>MRIPLVGKDSIESKDIGFTLIHEHLRVFSEAVRQQWPHLYNEDEEFRNAVNEVKRAMQFGVKTIVDPTVMGLGRDIRFMEKVVKATGINLVAGTGIYIYIDLPFYFLNRSIDEIADLFIHDIKEGIQGTLNKAGFVKIAADEPGITKDVEKVIRAAAIANKETKVPIITHSNAHNNTGLEQQRILTEEGVDPGKILIGHLGDTDNIDYIKKIADKGSFIGLDRYGLDLFLPVDKRNETTLRLIKDGYSDKIMISHDYCCTIDT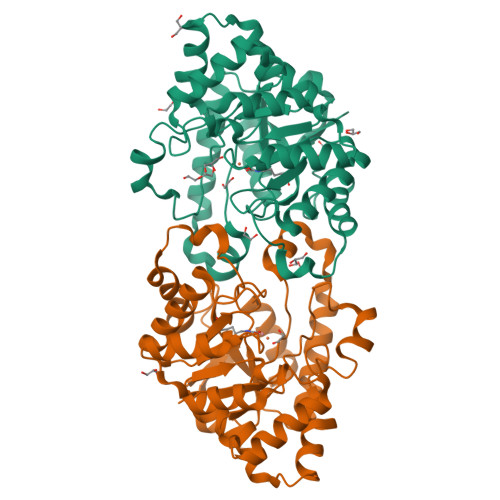GTAKPEYKPKLAPRWSITLIFEDTIPFLKRNGVNEEVIATIFKENPKKFFS[4x]N-[(piperidin-4-yl)methyl]methanesulfonamide 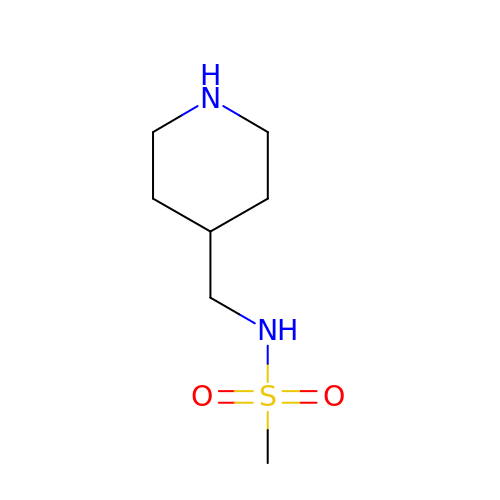| C7 H16 N2 O2 S | LULUGSQUPICPQM-UHFFFAOYSA-N> MC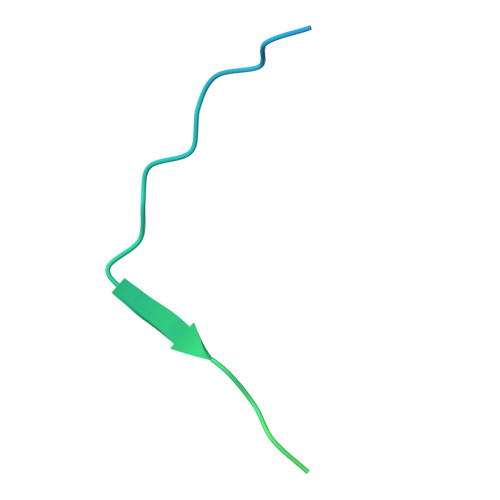FSPKISTPKPSVQAPEPAPLSEEVASVDIGAESDVDTNETKGIKDLKVKKESAPKDKSSVSRAMRNSGVNMG> RAGPVTW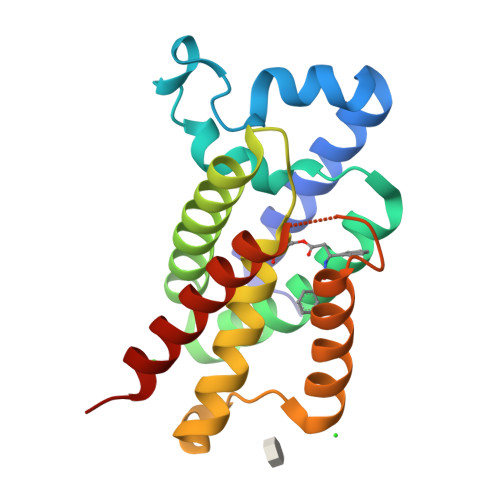VMMIACVVVFIAMQILGDQEVMLWLAWPFDPTLKFEFWRYFTHALMHFSLMHILFNLLWWWYLGGAVEKRLGSGKLIVITLISALLSGYVQQKFSGPWFGGLSGVVYALMGYVWLRGERDPQSGIYLQRGLIIFALIWIVAGWFDLFGMSMANGAHIAGLAVGLAMAFVDSLN>MASPRELTQNPLKKIFMPYSNGRPALHASQRGVCMTNCPTLIVMVGLPARGKTYISKKLTRYLNFIGVPTREFNVGQYRRDMVKTYKSFEFFLPDNEEGLKIRKQCALAALNDVRKFLSEEGGHVAVFDATNTTRERRAMIFNFGEQNGYKTFFVESICVDPEVIAANIVQVKLGSPDYVNRDSDEATEDFMRRIECYENSYESLDEEQ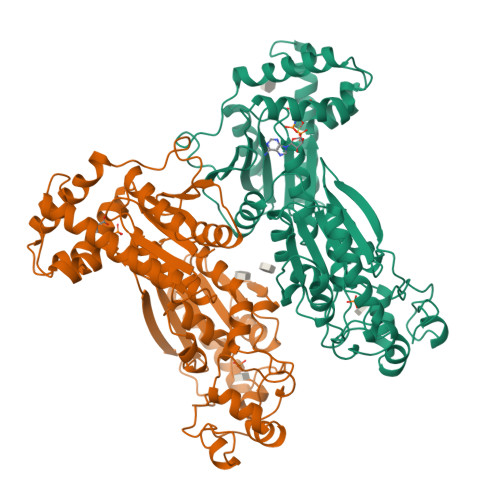DRDLSYIKIMDVGQSYVVNRVADHIQSRIVYYLMNIHVTPRSIYLCRAGESELNLKGRIGGDPGLSPRGREFSKHLAQFISDQNIKDLKVFTSQMKRTIQTAEALSVPYEQFKVLNEIDAGVCEEMTYEEIQDHYPLEFALRDQDKYRYRYPKGESYEDLVQRLEPVIMELERQENVLVICHQAVMRCLLAYFLDKAAEELPYLKCPLHTVLKLTPVAYGCKVESIFLNVAAVNTHRDRPQNVDISRPSEEALVTVPAHQ[2x]> SANNPWTGFQIFLSPYYANEVAAAAKQITDPTLSSKAASVANIPTFTWLDSVAKIPDLGTYLASASALGKSTGTKQLVQIVIYDLPDRNCAAKASNGEFSIANNGQANYENYIDQIVAQIQQFPDVRVVAVIEPDSLANLVTNLNVQKCANAKTTYLASVNYALTNLAKVGVYMYMDAGHAGWLGWPANLSPAAQLFTQVWQNAGKSPFIKGLATNVANYNALQAASPDPITQGNPNYDEIHYINALAPL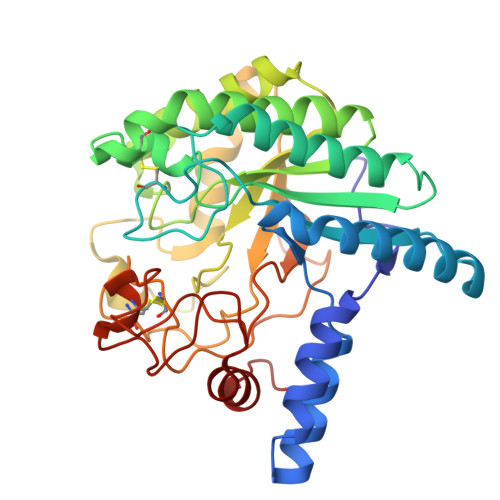LQQAGWDATFIVDQGRSGVQNIRQQWGDWCNIKGAGFGTRPTTNTGSQFIDSIVWVKPGGESDGTSNSSSPRYDSTCSLPDAAQPAPEAGTWFQAYFQTLVSAANPPL>GSHMQALSTRTAKNTL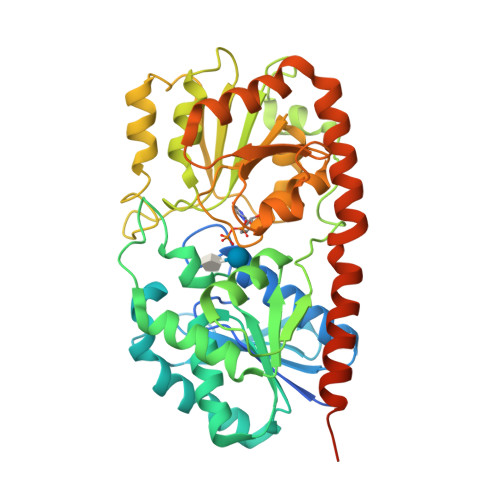PRAFAMPQPQVPARQPIALISVHGDPAADVGHESAGGQNIYVRQLGEALAAAGWHVDMFTRKTDPNDPDVIEHSPHCRTIRLQAGPLTYIPREKLFETLPKFVEAFKAYHAKYGYPLIHTNYWLSGWVGWQLRQQFNFQWLHTYHSLGVVKYQVASEQAQRDETRLMVEKAILENADCVIVTSPQEEAYLRRWVSKAGQTRLIPCGTNLKLFYPVADARAQLNLPADEPIVLYVGRFDRRKGIETLVAAMAQIPQGQLLLVGGSDPQRSDGAERRRIEGLVQEYNLGDRVTFVGQIDHEYLAVYYSAANVCVVPSYYEPFGLVAIEAMACGTPVIASAVGGLQFTVIPEETGLLVPPQDANALANAIQRILADPAWARTLGKNGRERVQALFNWEAIALQMGQLYRQLFAASLMGNSPRLEMVKNTASLAAVTKAALAS[12x]> HHWESKFSKEGLTFDDVLLVPAKSEVLPRDVDLSVELTKTLKLNIPVISAGMDTVTESAMAIAMARQGGLGIIHKNMSIEQQAEQVDKVKRSERGITNPFFLTPDHQVFDAEHLMGKYRISGVPIVNNEEDQKLVGIITNRDLRFIADYSMKISDVMTKEELVTASVGTTLDEA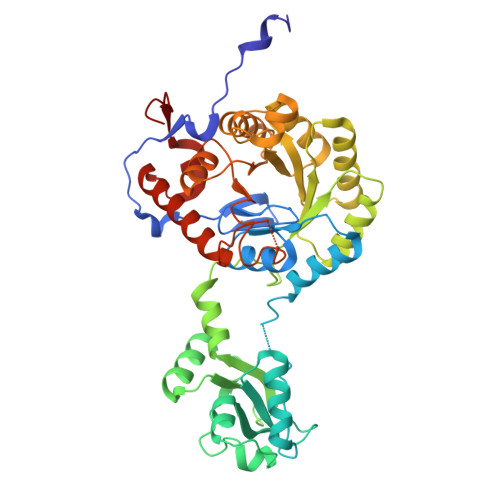EKILQKHKIEKLPLVDDQNKLKGLITIKDIEKVIEFPNSSKDIHGRLIVGAAVGVTGDTMTRVKKLVEANVDVIVIDTAHGHSQGVLNTVTKIRETYPELNIIAGNVATAEATRALIEAGADVVKVGIGPGSICTTRVVAGVGVPQITAIYDCATEARKHGKTIIADGGIKFSGDITKALAAGGHAVMLGSLLAGTSESPGAAAAPYKGPVEETVYQLVGGLRSGMGYCGSKDLRALREEAQFIRMTGAAA> MKRQGKRPSKNLKARCSRKALHVNFKDMGWDDWIIAPLEYEAFHCEGLCEFPLRSHLEPTNHAVIQTLMNSMDPESTPPTCCVPTRLSPISILFIDSANNVVYKQYEDMVVESCGCR;> ETGQCRIQKCTTDFVSLTSHLNSAVDGFDSEFCKALRAYAGCTQRTSKACRGNLVYHSAVLGISDLMSQRNCSKDGPTSSTNPEVTHGTKHHHHHH

Repulsive guidance molecules (RGMs) are cell surface proteins that control processes ranging from brain development to iron metabolism. RGMs can bind to the cell guidance receptor Neogenin (NEO1) and act as coreceptors for the bone morphogenetic proteins (BMPs). Structural analysis of RGMs and their complexes with NEO1 and BMP2 revealed a common RGM architecture comprising an N-terminal domain (RGMND) essential for BMP binding and a C-terminal domain (RGMCD) sufficient for NEO1 binding. Here, we determined high-resolution structures of all three human RGMs in complex with the BMP ligand growth differentiation factor 5 (GDF5) and the ternary complex of GDF5 with RGM and NEO1.

The RGMB–GDF5 interface is mainly formed by two interaction sites. First, a short linker between helices α2–α3 harbors the “RGD-loop” in RGMA and RGMC (“RGN” in RGMB) and interacts with the GDF5 wrist region. Second, the RGMB α3 helix stretches across the two GDF5 fingers. Under these conditions the RGMB ectodomain (RGMBECD) bound GDF5 with an apparent affinity (Kd) of 8.8 μM, and the N-terminal domain alone (RGMBND) exhibited a Kd of 2.7 μM, suggesting that RGMBND comprises the major domain for GDF5 binding. Mutations of RGMB at either of two key RGMB–GDF5 interactions (Leu103Glu and His106Arg) abolished binding to GDF5. In solution the 2:2 RGMB–GDF5 complex is stable at pH 7.5, but dissociates at pH 5.5, similarly to the RGMB–BMP2 complex.>GPQDPDKRRKTLVIIEKTYSLLLDVEDYERRYLLSLEEERPALMDDRKHKICSMYDNLRGKLPGQERPSDDHFVQIMCIRKGKRMVARILPFLSTEQAADILMTTARNLPFLIKKDAQDEVLPCLLSPFSLLLYHLPSVSITSLLRQLMNLPQSAATPALSNPHLTAVLQNKFGLSLLLILLSRGEDLQSSDPATESTQNNQWTEVMFMATRELLRIPQAALAKPISIPTN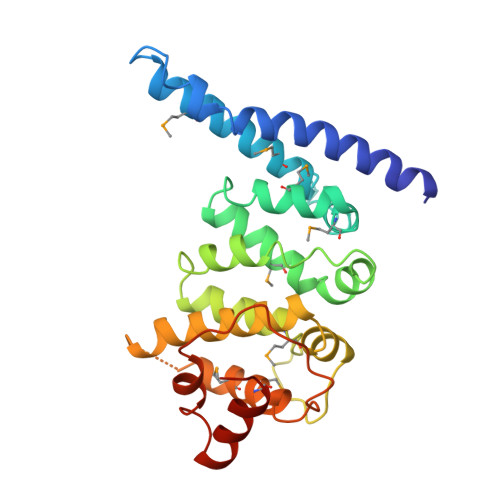LVSLFSRYVDRQKLNLLETKLQLVQ[4x]>[4x]MTLLTNAEEIS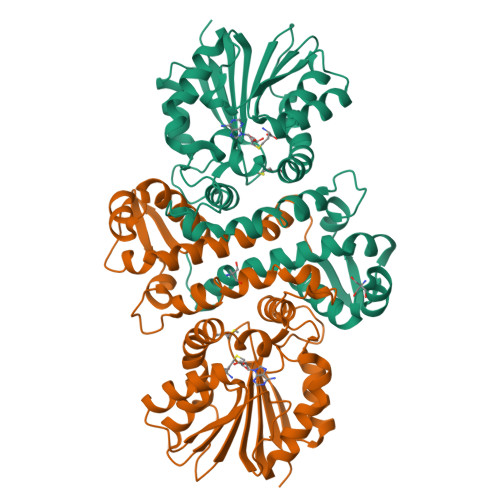DIAFGFMGSKALFAALHHGVFTCLADGPLSVEEMAAATGLHPDRVQTLLTALASLGVVSAVEGRFANSPAAESFLVKGAKYDFGDYLRLQVDRQMYGLLDQIEDAIANNLPDDATSSYADWFSDPEQAKLYSNSQHAGSLGPARGLAKLIDLSGGKKLLDVGGGTGAFAITLCKAFADLAATIVDFPNVAALGKGYVEKAGLSDRIEYVIGDALRTEWPREQDAILMSYLFSGVAGDEHDSLLKRAYDHLVPGGRLLIHDFVVTADRTGPKLAALWQLQHTAFTPEARSLDDEWLAEQLKKTGFTDVKVGPMIPGMTMLAEAVRPEHHHHHH>EFSRKTYTLTDYLKNTYRLKLYSLRWISDHEYLYKQENNILVFNAEYGNSSVFLENSTFDEFGHSINDYSISPDGQFILLEYNYVKQWRHSYTASYDIYDLNKRQLITEERIPNNTQWVTWSPVGHKLAYVWNNDIYVKIEPNLPSYRITWTGKEDIIYNGITDWVYEEEVFSAYSALWWSPNGTFLAYAQFNDTEVPLIEYSFYSDESLQYPKTVRVPYPKAGAVNPTVKFFVVNTDSLSSVTNATSIQITAPASMLIGDHYLCDVTWATQERISLQWLRRIQNYSVMDICDYDESSGRWNCLVARQHIEMSTTGWVGRFRPSEPHFTLDGNSFYKIISNEEGYRHICYFQIDKKDCTFITKGTWEVIGIEALTSDYLYYISNEYKGMPGGRNLYKIQLSDYTKVTCLSCELNPERCQYYSVSFSKEAKYYQLRCSGPGLPLYTLHSSVNDKGLRVLEDNSALDKMLQNVQMPSKKLDFIILNETKFWYQMILPPHFDKSKKYPLLLDVYAGPCSQKADTVFRLNWATYLASTENIIVASFDGRGSGYQGDKIMHAINRRLGTFEVEDQIEAARQFSKMGFVDNKRIAIWGWSYGGYVTSMVLGSGSGVFKCGIAVAPVSRWEYYDSVYTERYMGLPTPEDNLDHYRNSTVMSRAENFKQVEYLLIHGTADDNVHFQQSAQISKALVDVGVDFQAMWYTDE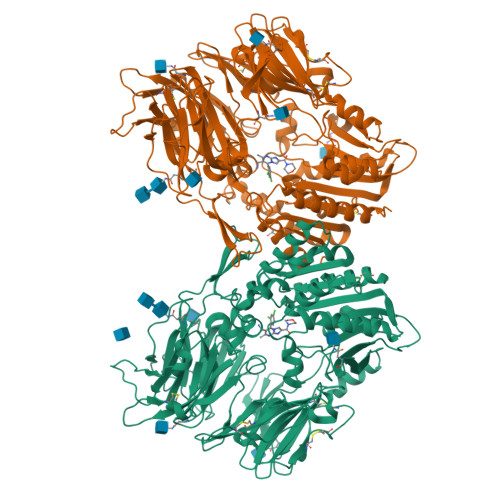DHGIASSTAHQHIYTHMSHFIKQCFSLPPLEQKLISEEDLNSAVDHHHHHH[2x]>[4x]MYGSKTFIKYVSGIPDYFKQSFPEGFTWERTTTYEDGGFLTAHQDTSLDGDCLVYKV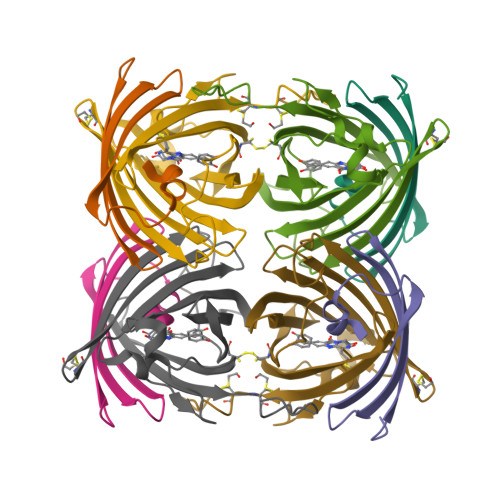KILGNNFPADGPVMQNKAGGWEPGCEILYEVDGVLCGQSLMALKCPGGRHLNCRLHTTYRSKKPASALKMPEFHFEDHRIEVKEVQKGKHYEQYEAAVARYCDAAPSKLGHH;>MASLLTETMPFRMTMEGTVNGHHFKCTGKGEGNPFEGTQDMKIEVIEGGPLPFAFDILSTSC[4x]>MRGSHHHHHHGRSRSLNPLSTPQFDSTDETPASYNLAVRRAAPAVVNVYNRGLNTNSHNQLEIRTLGSGVIMDQRGYIITNKHVINDADQIIVALQDGRVFEALLVGS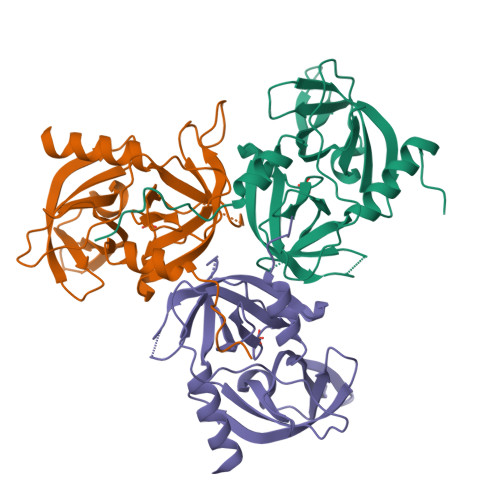DSLTDLAVLKINATGGLPTIPINARRVPHIGDVVLAIGNPYNLGQTITQGIISATGRIGLNPTGRQNFLQTDASINHGNSGGALVNSLGELMGINTLSFDKSNDGETPEGIGFAIPFQLATKIMDKLIRDGRVIR[3x]3-[(2S)-pyrrolidin-2-ylethynyl]pyridine 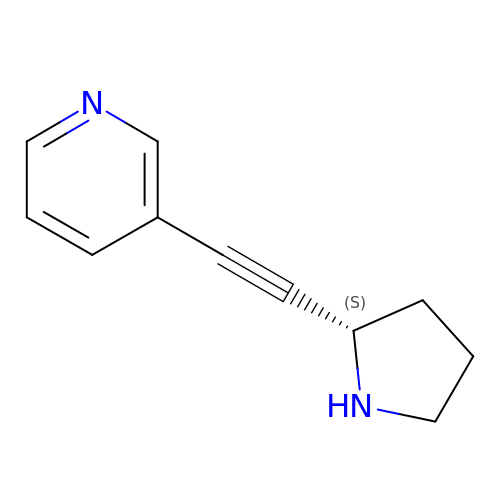| C11 H12 N2 | YOOCTKCKTOXZCT-NSHDSACASA-N>[6x]MMAYNKEEKIKSLNRMQYEVTQNNGTEPPFQNEYWDHKEEGLYVDIVSGKPLFTSKDKFDSQCGWPSFTKPIEEEVEEKLDTSHGMIRTEVRSRTADSHLGHVFNDGPGPNGLRYCINSAALRFVPKHKLKEEGYESYLHLFNK

Oxidation of Met to methionine sulphoxide (Met-SO) damages the proteins and can alter protein function. However, these damaged proteins can be reversed by the repair enzymes, methionine sulphoxide reductases (Msr). Two distinct Msr enzymes have been classified for the reduction of Met-SO: MsrA reduces the S-form of Met-SO and MsrB reduces the R-form. However, enzymatic studies demonstrate that both the enzymes share a common catalytic mechanism based on sulphenic acid chemistry involving two (or three) cysteine residues.

Our crystal structure of BsMsrB was found to be identical to the NMR BsMsrB structure and was further used for structure comparison. The specific activity of BsMsrB was slightly lower than the MsrB activity of SpMsrAB and of mammalian MsrBs. BsMsrB also has a low Km value, similar to that of SpMsrAB for dabsyl-Met-R-SO.> MVEQMLSKNMLLGGFDTGNIKAKISFLNEKGNI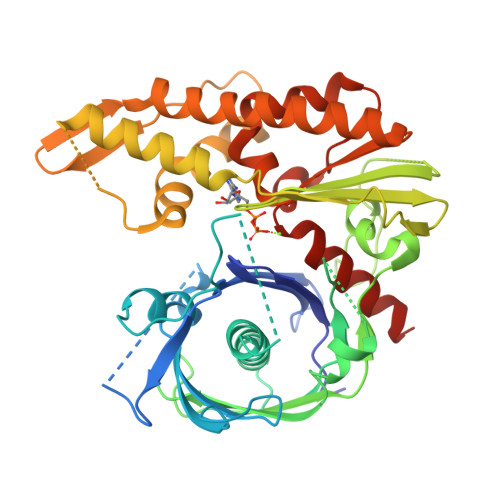ESFAIPTVIAEAPPAKIDLKSAPSKKNDYVNEKDEDIELLHVRIISNSLDGDARSRAWYVGAYAKDQEDRQEPTVDEMGKTEDKFSQKNKKLHLIPLFTSMAVAAARIGKEEVSVPFSGGMPIEDYKLRGEEQILEMLYGEHTVEFLDGTYEGKKIKITINDGTMNVEGVSSVLAILFDIVNGEIVEVEGMDAEIGESYAINDLGAGTSDNAFFEDGELNKKLSTNTDLGTNKYIDEILKNIKERFMENEILKSFMTDEIESPFKTREDFIQRLVMPEVEKMIEDDTYKPTFSVKWGPVKENVTDIVMDGMLKYAEDQKASLDKFWDKTNADKNIVVGGGVLFGYAGLRDLKEQDGFILPKNIQESAYFTSRSYLIANLLEQLNKEGVEA>MPNIVLFSGSSHQDLSQRVADRLGLELGKVVTKKFSNQETSVEIGESVRGEDVYIIQSGCGEINDNLMELLIMINACKIASSSRVTAVIPCFPYARQDKKDKSRAPISAKLVANMLSVAGADHIITMDLHASQIQGFFDIPVDNLYAEPAVLQWIRENIAEWKNCIIVSPDAGGAKRVTSIADRLNVEFALIHKERKKANEVDRMVLVGDVKDRVAILVDDMADTCGTICHAADKLLSAGATKVYAILTHGIFSGPAISRINNAAFEAVVVTNTIPQEDKMKHCTKIQVIDISMILAEAIRRTHNGESVSYLFSHVPLHHHHHH[6x]

PRPP synthase (PRPS) transfers the pyrophosphate groups from ATP to ribose-5-phosphate to produce 5-phosphate ribose-1-pyrophosphate (PRPP), a key intermediate in the biosynthesis of several metabolites including nucleotides, dinucleotides and some amino acids. Although hPRPS1 and hPRPS2 share 95% sequence identity, hPRPS2 has been shown to be less sensitive to allosteric inhibition and specifically upregulated in certain cancers in the translational level. As a rate limiting enzyme, the regulation of PRPS is very complex. hPRPS uses ATP or dATP as pyrophosphate donor and can be allosterically regulated by inorganic phosphate Pi and ADP.

Here, we find that hPRPS2 can form filaments in vitro, and the structure of hPRPS2 is obtained by cryo-EM with 3.08A resolution. The twist and rise of hPRPS2 filament are 30° (left-handed twist) and 63 Å, respectively. The hexamer of hPRPS2 had D3 symmetry, there were 6 active sits (ATP and R5P binding site)and 6 allosteric sites in a hPRPS2 hexamer. Here, we solve the human PRPS2 filament structure with ADP binding in ATP site and allosteric site 1 and Pi binding in the R5P site. The ADP in the active site can interact with three monomers, which means hPRPS2 needs to be assembled properly to function. ADP in allosteric site also interacts with 3 monomers, and it formed hydrogen bond with regulatory flexible loop (RF loop Y94-S108). Each interaction site contains some identical amino acids. hRPPS2 hexamers are connected by salt bridges formed between R301 and E298 pairs, the hydrogen bonds between R301, N305, and E307, and also the van der Waals’ Forces between R302 and R301. When incubated with allosteric regulator ADP and Mg2+, or ATP, R5P, phosphate and Mg2+, or PRPP, phosphate and Mg2+, hPRPS2 could form long filaments, and the mutant hPRPS2R301A and hPRPS2R302A lost its filament-forming ability. The enzyme activity results showed that the mutant hPRPS2R301A and hPRPS2R302A almost lost its activity. K99 in the RF loop may be a key amino acid residue related to the allosteric inhibition of ADP.1-(3-AMINO-1,2-BENZISOXAZOL-5-YL)-6-(2'-{[(3R)-3-HYDROXYPYRROLIDIN-1-YL]METHYL}BIPHENYL-4-YL)-3-(TRIFLUOROMETHYL)-1,4,5,6-TETRAHYDRO-7H-PYRAZOLO[3,4-C]PYRIDIN-7-ONE | C31 H27 F3 N6 O3 | 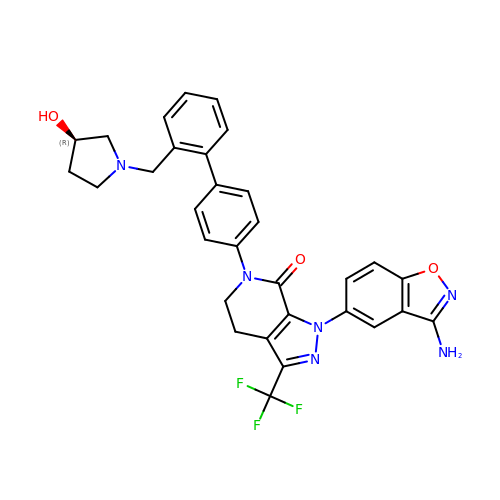DFRIQJHMGZBFOM-JOCHJYFZSA-N> MSAPPNTLFLRLEGALQSWGSNEAKFALRRTADAPTKSGVLGLLCAAMGIGRAEAADSWLPKLANLRMGVRIDRPGIRWWDFHTVGAGQRMRMAELKAPKKPSMVGAALAETLTPSKVKTRAETLLSRREYLADASFLVALQGEPELVAKLSAALAKPVWAIYLGRKSCPPSRPVCEHPPGFYNTLEEALSAVPLQKRWHNEPLPQILPCVMDWIPGYDGEHAPDDAEIHYDLPVSFQPPRHLPRFVIRRELVVGEDVQVSRETGTSVWRPKGTRADYNNSEYKKVRAERLVMDHAACMVCKAPATTVQHVNYRRAGGKEIPEDLRALCRLCHDACTMLEYGSGMTTNRIDPCDPIWRERILAKRKEIVEFRSRGQRFRKMKPEEENG;> MIYLSRLLIDTGGNPDRPRPGRKWLDNIYNVHRRLSMAFPSGLRREQDPHFLKPFSPNDFQKTPFLFRVDNNIDGNDKRAIIIVQSVLEPDWDYCFQNALDFLAAPPETKEYNPEFKAGQLLRFRLRVNASVRRHIPEMVQQDGQTIETGKILHKRVSLTWDASSTPDQALADWLAAKSPKLGFTLQRCELLQLGWVYGSKPEPKNVKVKEQGQGYWREHKYNPLRFRAALLEGVLEVDDPKLFLKTLSSGIGKAKSFGFGLLSVLPIRNDG;>[6x]MLIEIHMIQNHSPANLNRDDLGAPKTCYFGGVLRSRISSQCIKRSIRTSNDFKALLGGVRTRRLADLIQQEAG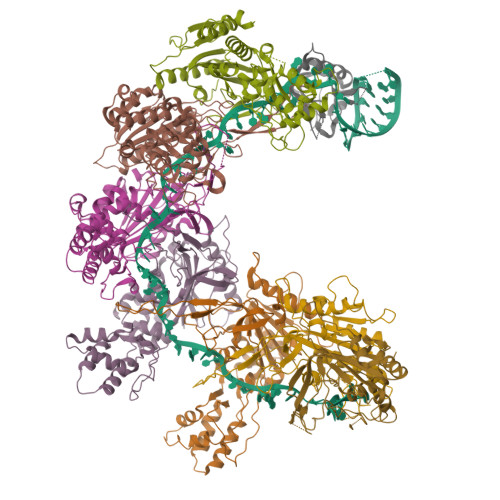ETECWKKAQEILNKCGFKNKDDNTKMLVFMSKDKIKDLARIVLDNSLGLTEAAQQVANVIAQATLAPDIALCGRMLEPNDKDKDKKVKWSNTTVEAALQVAHAISTHIARPEIDYFVAADDVPGEDAGAGHIGESMFASACFYKYFSIDWEQLVKNLKGDTNLAAHTVGAFLLAAAKTNPSGKQNSFAAHNYPDGILVEFKNSPISYANAFVRPVSVVKESDLVEQSIGQLSNYVNDIRLGYYDEQSPVIGFWFSPNNRYPLGYKHSKLASRNIGNLNELVGAVLDYIGGFKWEEVQKSKAYIGG>[2x]GEFMEEGKMDENEWSYHGEGNKSLVVAHAQRCVVLRFLKFPPNKKKTSEEILQHLQNIVDFGKNVMKDFLGENYVHCGEVVQLPLEFVKQLCLKIQCERPESRCDKDLDTFSGYAMCLPNLTRLQTFHFAEHRPILCVEIKPKCGFIPFSNDVTHEMKHKVCRYCMHQHLKVATGKWKKISKYCPLDLYSGNKQRMHFALRSLLQETQNNLRIFKNGELIYGCGDARSPVADLKELAHHLKPFFFPSNGLASGPHCTKAVIRELVHVITRVLLSSSEKARAGALRLGLQGPRVCEASPFSRSLHNQGKNTSEHSGLPKGCLLYKTLQVQMLDQLDIEGLYPLYKRVEQYLEEFPEERKTLQIDGPYDEVFYQKLLDLSTEDDGTVAFALTKVQQYRVAMTAKDCSIMIALSPCLQGTSSDQRPVIPSSRSRLAFSVSVLDLDLKPYESIPHQYKLDSKIVNYYSKTVHAKD

Inositol 1,3,4,5,6-pentakisphosphate 2-kinase (IP5 2-K)3 is a key enzyme of higher inositol phosphate (inositide, IP) metabolism. IP5 2-K is present in yeast to mammals and catalyzes the synthesis of phytic acid (inositol hexakisphosphate or IP6) from IP5 and ATP. Mouse IP5 2-K folds in two lobes, N- and C-terminal lobes, connected by a hinge, thereby conserving the general fold scheme of PKs and IPKs, and in a similar way, both lobes coordinate the nucleotide between them. The CIP lobe represents more than half of the protein and is specific to IP5 2-K enzymes.

In addition, we present two different crystal forms, including one or two molecules in the asymmetric unit, respectively, the first showing much better resolution (2.4 versus 3.2 Å). mIP5 2-K presents two zinc ions in its structure, one in the CIP-lobe (Zn1) and the other close to the hinge region (Zn2). In fact, Zn1 is present in all the crystals obtained, whereas Zn2 was only detected in the low resolution ΔC-mIP5 2-K crystals in which the two molecules in the asymmetric unit interact through the hinge region probably fixing a conformation captured by crystallography. Regarding Zn2, it is created by two residues from the hinge (His-125 and His-129) and one residue from the C-lobe (Cys-410). Mutation of residues His-129 and Cys-410 to serine produces samples with a moderate decrease in enzymatic activity revealing that Zn2 is not critical for protein function. Therefore, Zn1 is key in all mammal IP5 2-K enzymes, whereas Zn2 could be an artifact of crystallization. Unexpectedly, the formation of the ternary complex (mIP5 2-K + IP5 + ATP) was achieved by protein incubation with IP6 and ADP.> MEGEKGSKTRKGDALAREKLLEIAEKIYNQFEEEVVPSVSLPSRTKANLEYSDESDVWVYGDRESERSAKTVKGAFQLLKTTYATDFLINEHLARNRGSTLRELYYISEGWDYAKFKEQGESDRLIEDLEILTSLQREYFHMRPEEDGATMFGPIEITEQTKRGERNIHCQKDVGEGGYQIPFNVENIEFQKHDASMIIAIETGGMYARLMENGFDEAYNAILVHLKGQPARSTRRIIKRMNEELGIPVAVFTDGDPWSYRIYASVAYGAIKSAHLSEFMATPAAKFLGLQPSDIVEYELSTDKLTEQDVSALRSELSDPRFESDYWKEQIQLQLDIGKKAEQQAFAGKGLDFVTEVYLPNRLKEMGMI;> METPIAEELAKKQKSISVAEFFEKNRQILGFDSAPRSLITTVKEAVDNALDACEEAGILPDILVQVERTGPDYVTVIIEDNGPGIVREQIPKVFAKLLYGSRFHALKQSRGQQGIGISAAVLYAQMTAGRHTKILSKTSPTAPAHYYELMINTSTNEPDILVDEVRDWFRPHGTQIELEMRAAYVKGRRQSIYEYLKATAIVNPHARITLIDPDGNEEVFERATDKMPEPAEEILPHPEGIELGTLMKMLHYTERQKLAPFLRYSFCKIGLLTAEEICKAAGLDPEIDPHALGRHEARKLIEAFEKVKIMAPPTDCLSPIGEDLIYRGLEKETTVDFIATSTRKPAVYSGNPFVVEVGMAYGGNLPKEEKISIMRFANRVPLLYQQGGCVTTHAVEDIKWKQYGLNQPGGGIPVGPVILLIHVASINVPFTSESKDAIADIPVIKEEIDLAIKEVARKLKHYLSKQS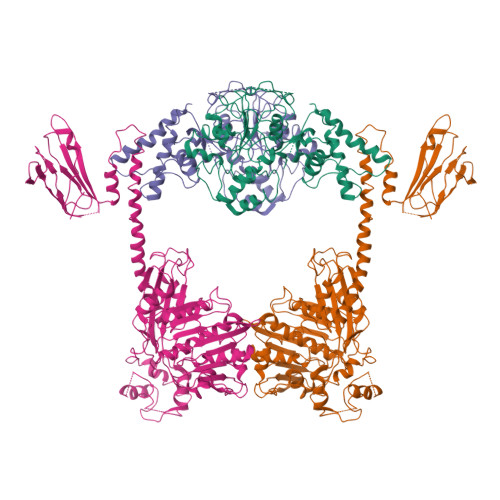NLKKRREKEIIITKVLPKLAAKVAHVLEKDVPDINPVVAKIMGNLLVHRVIKNNGDGTVDVAIKVKNFGTSAYSFRVHEMLPCKVSGAKPEPKVVTMGNDYDYVWDISASAGSSKVLSYKIESASEEELQKLPQLIVEGIEEELVTGAKAFKGV Enolase, a ubiquitous enzyme, catalyzes the reversible conversion of 2-phospho­glycerate (2PG) to phospho­enolpyruvate (PEP) in the glycolytic pathway of organisms of all three domains of life. Here we present structural snapshots of Mycobacterium tuberculosis (Mtb) enolase in apo, PEP-bound and two 2PG-bound forms as it catalyzes the conversion of PEP to 2PG. MtEno has a topology similar to other enolase structures, a smaller N-terminal domain and a larger C-terminal domain. The crystal and the cryoEM structures (enzyme in solution, frozen) along with the biochemical studies clearly demonstrate that the functional unit of MtEno is an octamer.

Of the two structures of MtEno-2PG, one harbored the 2PG-canonical pose. MtEno–PEP-canonical [Figs. 3(d) and 3(e)] and MtEno–2PG-canonical [Figs. 3(f) and 3(g)] have similar orientations of the bound ligand. In both of these structures, MgA 2+ coordinates with the carboxyl groups of Asp241, Glu283 and Asp310; a water molecule; and the carb­oxy­lic group of 2PG/PEP. However, MgB 2+ coordinates weakly with the carb­oxy­lic and phosphate moieties of 2PG/PEP, the β-OH group of Ser42, and water molecules [Figs. 3(e) and 3(g)]. Hydrogen-bonding interactions with Arg364 in the highly conserved loop 4 further stabilize the associations via the phosphate moiety. Additionally, the carboxyl­ate group of 2PG/PEP interacts with both Mg2+ ions and residues Glu163, Lys386, Asp310 and Lys335 of the enzyme. Notably, 2PG in this alternate conformation has fewer hydrogen-bonding interactions in the active site due to the absence of catalytic MgB 2+. MgB 2+ plays an important role in the closing of active site loop 1 and the neutralization of the negative charge of the phosphate group in 2PG-canonical [Fig. 3(i)]. The motions of these loops are subtle in the PEP-bound state, and although the overall structure resembles to that of the apo state of MtEno, the active site loops are partially closed in the presence of PEP. The two 2PG-bound structures depict closed active site loops and more pronounced deviations in loop 2, up to 5.2 Å as in the case of Asp156 [Figs. 3(b) and 3(c)]. MtEno–PEP-canonical and MtEno–2PG-canonical possess negative binding free energy values of −5.6 and −29.9 kcal mol−1, respectively.

>MHHHHHHMPIIEQVRAREILDSRGNPTVEVEVALIDGTFARAAVPSGASTGEHEAVELRDGGDRYGGKGVQKAVQAVLDEIGPAVIGLNADDQRLVDQALVDLDGTPDKSRLGGNAILGVSLAVAKAAADSAELPLFRYVGGPNAHILPVPMMNILNGGAHADTAVDIQEFMVAPIGAPSFVEALRWGAEVYHALKSVLKKEGLSTGLGDEGGFAPDVAGTTAALDLISRAIESAGLRPGADVALALDAAATEFFTDGTGYVFEGTTRTADQMTEFYAGLLGAYPLVSIEDPLSEDDWDGWAALTASIGDRVQIVGDDIFVTNPERLEEGIERGVANALLVKVNQIGTLTETLDAVTLAHHGGYRTMISHRSGETEDTMIADLAVAIGSGQIKTGAPARSERVAKYNQLLRIEEALGDAARYAGDLAFPRFACETK[4x]>[2x]XGELK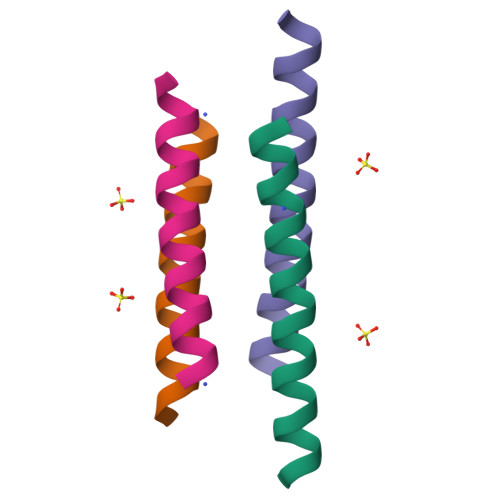AIAQELKAIAKELKAIAWEEKAIAQGX> MTVATATDSTITKSDFEKQLKDRYGKDMLYEMIAQDVITKKYKVSDDDVDKEVQKAKSQYGDQFKNVLKNNGLKDEADFKNQIKFKLSMNKAIKQSVTEKDVKDHYKPEIKASHILVSDENEAKEIKKKLDTGASFEELAKQESQDLLSKEK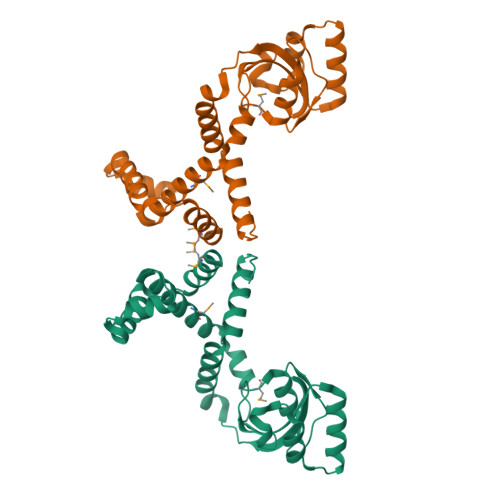GGDLGYFHSGAMTPEFETAAYKLKIGQISDPVQSPNGYHIIKLTGKKDLKPYDEVKNSIRKNLEEERTADPIFGKKLLQSELKKANIKINDSELEDTFTIVSPQGNENLYFQ oxo(propan-2-ylamino)acetic acid | 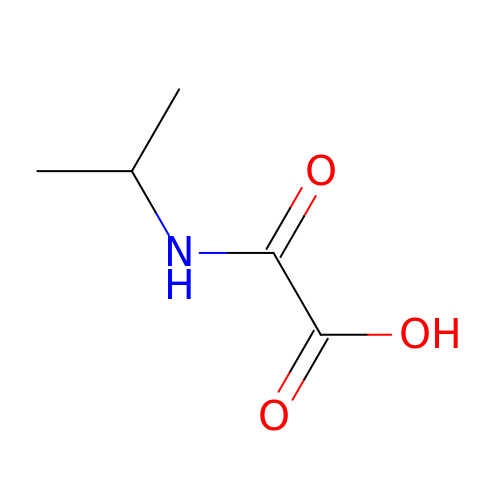C5 H9 N O3 | KBMFHCMLHQGQEB-UHFFFAOYSA-N> SRPHQWQTDEEGVRTGKCSFPVKYLGHVEVDESRGMHICEDAVKRLKAERKFFKGFF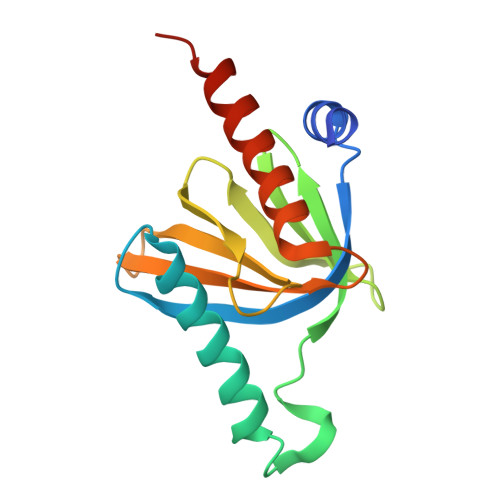GKTGKKAVKAVLWVSADGLRVVDEKTKDLIVDQTIEKVSFCAPDRNFDRAFSYICRDGTTRRWICHCFMAVKDTGERLSHAVGCAFAACLERKQKREKE>[3x]GGSGPKAQLMLRYPDGKREQITLPEQAKLL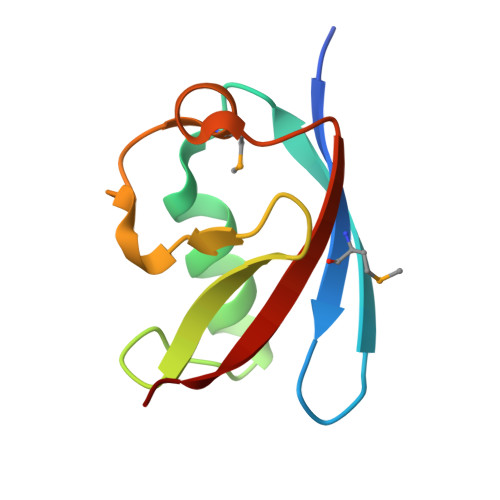ALVKHVQSKGYPNERFELLTNFPRRKLSHLDYDITMQEAGLCPQETVFVQERN> 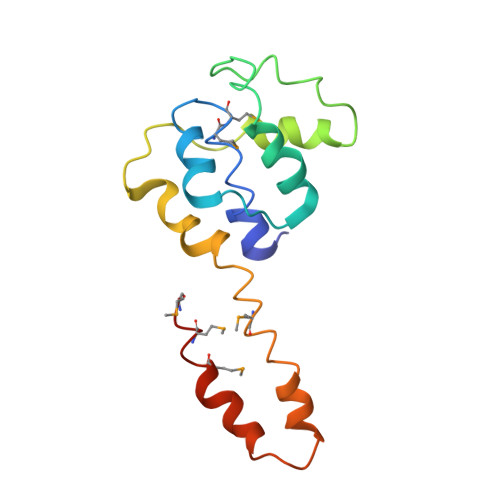KLLPAFQNAERLLLAHMMRSRDVALVVQERIGGRFNIEEHRALAAYIYAFYEEGHEADPGALISRIPGELQPLASELSLLLIADDVSEQELEDYIRHVLNRPKWLMLKVKEQEKTEAERRKDFLTAARIAKEMIEMKKMLSSS>[8x]GGQLV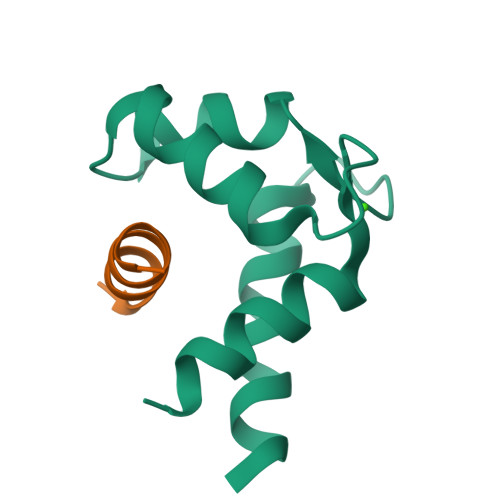MLRKAQEFFQTCDAEGKGFIARKDMQRLHKELPLSLEELEDVFDALDADGNGYLTPQEFTTGFSHFFFSQN;>NMKAGATSEGVLANFFNSLLSKKTG[8x]>[2x]MWFRNLLVYRLTQDLQLDADSLEKALGEKSARPCAS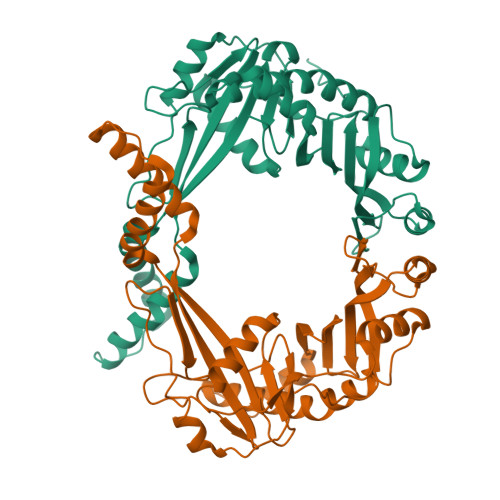QELTTYGFTAPFGKGPDAPLVHVSQDFFLISARKEERILPGSVVRDALKEKVDEIEAQQMRKVYKKERDQLKDEIVQTLLPRAFIRRSSTFAAIAPSLGLILVDSASAKKAEDLLSTLREALGSLPVRPLSVKVAPTATLTDWVKTQEAAGDFHVLDECELRDTHEDGGVVRCKRQDLTSEEIQLHLTAGKLVTQLSLAWSDKLSFVLDDKLAVKRLRFEDLLQEQAEKDGGEDALGQLDASFTLMMLTFAEFLPALFEALGGEEIPQGV>[4x]MSVLPFLRIYAPLNAVLAAPGLLAVAALTIPDMSGRSRLALAALLAVIWGAYLLQLAATLLKRRAGVVRDRTPKIAIDVLAVLVPLAAFLLDGSPDWSLYCAVWLLKPLRDSTFFPVLGRVLANEARNLIGVTTLFGVVLFAVALAAYVIERDIQPEKFGSIPQAMWWAVVTLSTTGYGDTIPQSFAGRVLAGAVMMSGIGIFGLWAGI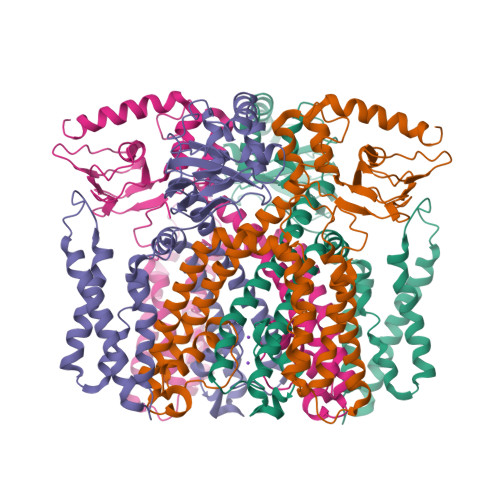LATGFYQEVRRGDFVRNWQLVAAVPLFQKLGPAVLVEIVRALRARTVPAGAVICRIGEPGDRMFFVVEGSVSVATPNPVELGPGAFFGEMALISGEPRSATVSAATTVSLLSLHSADFQMLCSSSPEIAEIFRKTALERRGAAASA> EWTGDSS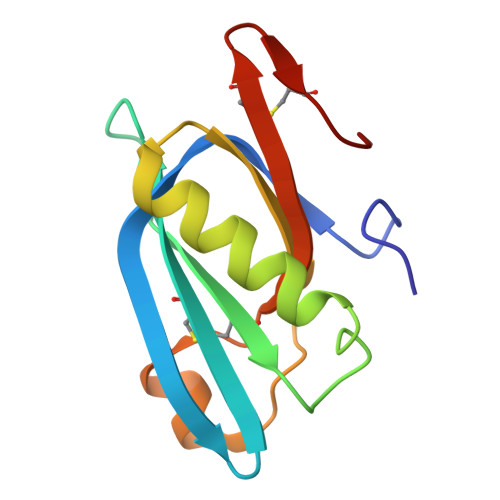INYYSDEVISDFHVGQFNRSAYFCIKTVKKSGEGTPIIACALSHDSKWIPSFNIMLEQARNFYITGHSIRVYVQPNVWSNKSFIEALSSNALVGLSSCSTSECFGPVKP benzaldehyde | C7 H6 O | 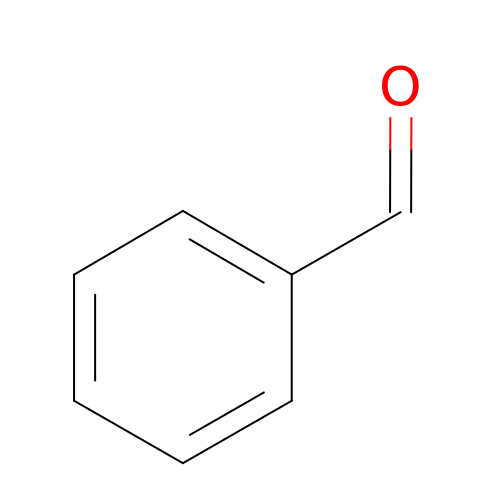HUMNYLRZRPPJDN-UHFFFAOYSA-N>GLELLIAQTILQGFDAQYGRFLEVTSGAQQRFEQADWHAVQQAMKNRIHLYDHHVGLVVEQLRCITNGQSTDAEFLLRVKEHYTRLLPDYPRFEIAESFFNSVYCRLFDHRSLTPERLFIFSSQPERRFRTIPRPLAKDFHPDHGWESLLMRVISDLPLRLHWQNKSRDIHYIIRHLTETLGPENLSKSHLQVANELFYRNKAAWLVGKLITPSGTLPFLLPIHQTDDGELFIDTCLTTTAEASIVFGFARSYFMVYAPLPAALVEWLREILPGKTTAELYMAIGCQKHAKTESYREYLVYLQGCNEQFIEAPGIRGMVMLVFTLPGFDRVFKVIKDKFAPQKEMSAAHVRACYQLVKEHDRVGRMADTQEFENFVLEKRHISPALMELLLQEAAEKITDLGEQIVIRHLYIERRMVPLNIWLEQVEGQQLRDAIEEYGNAIRQLAAANIFPGDMLFKNFGVTRHGRVVFYDYAEICYMTEVNFRDIPPPRYPEDELASEPWYSVSPGDVFPEEFRHWLCADPRIGPLFEEMHADLFRADYWRALQNRIREGHVEDVYAYRRRQRFSV[2x];>[2x]ESKVVVPAQGKKITLQNGKLNVPENPIIPYIEGDGIGVDVTPAMLKVVDAAVEKAYKGERKISWMEIYTGEKSTQVYGQDVWLPAETLDLIREYRVAIKGPLTTPVGGGIRSLNVALRQELDLYICLRPVRYYQGTPSPVKHPELTDMVIFRENSEDIYAGIEWKADSADAEKVIKFLREEMGVKKIRFPEHCGIGIKPCSEEGTKRLVRAAIEYAIANDRDSVTLVHKGNIMKFTEGAFKDWGYQLAREEFGGELIDGGPWLKVKNPNTGKEIVIKDVIADAFLQQILLRPAEYDVIACMNLNGDYISDALAAQVGGIG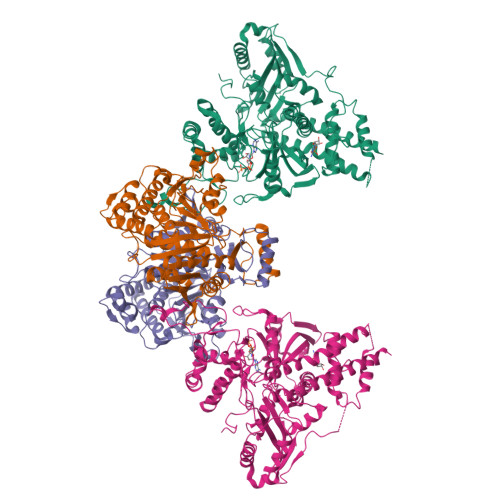IAPGANIGDECALFEATHGTAPKYAGQDKVNPGSIILSAEMMLRHMGWTEAADLIVKGMEGAINAKTVTYDFERLMDGAKLLKCSEFGDAIIENM>GHMSVSAFNRRWAAVILEALTRHGVRHICIAPGSRSTPLTLAAAENSA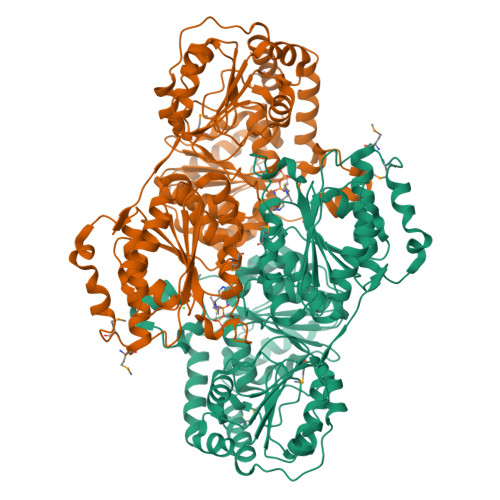FIHHTHFDERGLGHLALGLAKVSKQPVAVIVTSGTAVANLYPALIEAGLTGEKLILLTADRPPELIDCGANQAIRQPGMFASHPTHSISLPRPTQDIPARWLVSTIDHALGTLHAGGVHINCPFAEPLYGEMDDTGLSWQQRLGDWWQDDKPWLREAPRLESEKQRDWFFWRQKRGVVVAGRMSAEEGKKVALWAQTLGWPLIGDVLSQTGQPLPCADLWLGNAKATSELQQAQIVVQLGSSLTGKRLLQWQASCEPEEYWIVDDIEGRLDPAHHRGRRLIANIADWLELHPAEKRQPWCVEIPRLAEQAMQAVIARRDAFGEAQLAHRICDYLPEQGQLFVGNSLVVRLIDALSQLPAGYPVYSNRGASGIDGLLSTAAGVQRASGKPTLAIVGDLSALYDLNALALLRQVSAPLVLIVVNNNGGQIFSLLPTPQSERERFYLMPQNVHFEHAAAMFELKYHRPQNWQELETAFADAWRTPTTTVIEMVVNDTDGAQTLQQLLAQVSHL[4x]>GPAEKWKPTPAPTGTVAAAVTDTQVSKDNKFDDTKTLNNAGANGSLSNSKGNLGANIAAGSGNQQDNAAAITSSAGDAATVFAVADIYQESKDNKFTNKGTQNNALLNNSANNSSGNVGVNVAAGQGNQQKNNLAIVTADGKNVAAASNTEQVSLDNH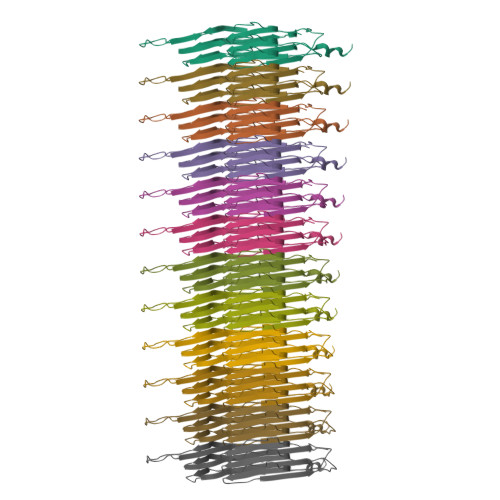FLNEASSKHSYKPQYVVNNAGLLNSANNASGNIGVNVAAGAGNQQSNTLTLGSGCTVCAAGTGSKLAF[12x]> MEDTARTDEQRRRVAGWTPVVKTLGDHRLRVAIVGRMNSGKSSLFNLLCEDPTMPAKKNIVKDFNGITRDCVEAHAALDDLHFTVIDTPGLLGGKLVEEAFRTVETADAAIFVTAVDEDVSAEEHDLIQYLAAKKMPTCLLVNKMDLVPEEEEALVLDVYNRLGLGKAVPFSARKREGLDMLSALLEPLYHIHAMRKVENDWDIEDLAMAGDEAAMEEIRDRNCTDRYIRVAIVGRTNSGKTSLVNRLVGYERNRAADESNTTRDPIEIACMYKGRKLKLIDTAGLARQRYRTDREFLSRIHSLSLNEIRYAHVVIVVFDATEGHPNKYDMSILHKVAQEGRPFVLCANKWDAVLDQSATAEAIDFKIKRQVQEVKYSNAVVVSAHTGMNLTLLMDQVLELYDTWNKRVRRSELT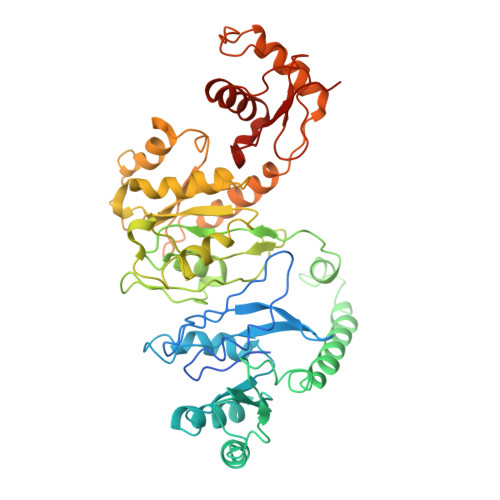KFWRKLEKSVIIPYHVARVGRITQISTRPPTFLLQLQTKKEESQLPKALQEMMKNAITEEFGFRGVPLRLVQEVKDSNPDYI>GSMAFVKSGWLLRQSTILKRWKKNWFDLWSDGHLIYYDDQTRQNIEDKVHMPMDCINIRTGQECRDT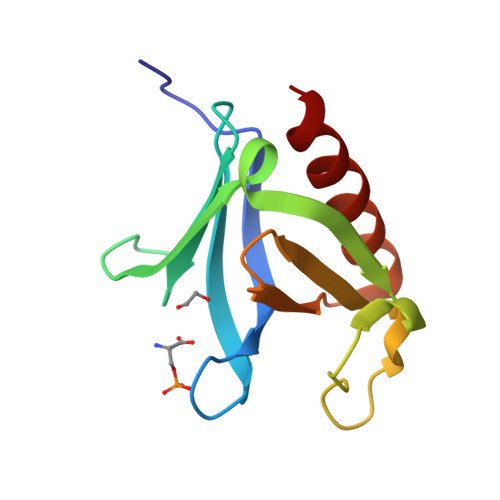QPPDGKSKDCMLQIVCRDGKTISLCAESTDDCLAWKFTLQDSRTN[2x]>GSAMGSEGLSDVASFATKLKNTLIQYHSIEEDKWRVAKKTKDVTVWRKPSEEFNGYLYKAQGVIDDLVYSIIDHIRPGPSRLDWDSLMTSLDILENFEENCCVMRYTTAGQLWNIISPREFVDFSYTVGYKEGLLSCGISLDWDEKRPEFVRGYNHPCGWFCVPLKDNPNQSLLTGYIQT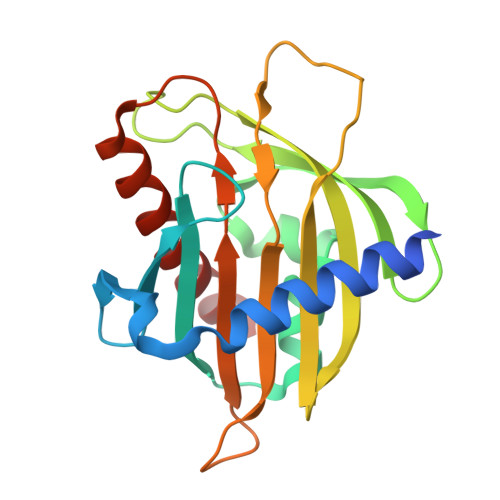DLRGMIPQSAVDTAMASTLTNFYGDLRKAL[2x]>GSHMSEQFDFDLERILKTIKDKNCKKVGLQFPEGLKRQAINIAREIEEKTRANVIISGNPCFGACDIDTILAGSVDILFHF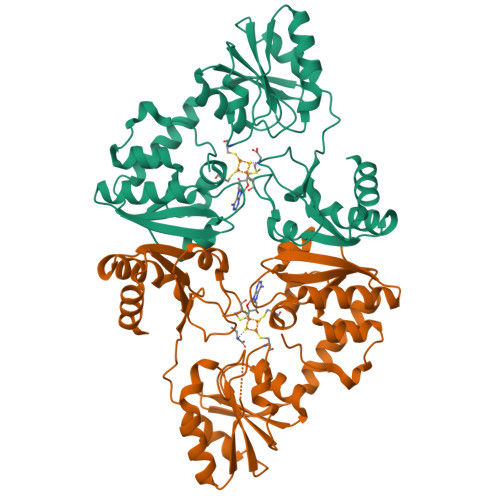GHAGMGEYENVVFIEARSNIDIIPAVKTALNLLKANRIGLITTVQHVHKLEEACKVIKEYGKECVIGKGDPRAIYPGQVLGCNFTAARVDCEEFIYIGSGIFHPLGVAIATKKRVIAADPFLNQAVEVSPERFLRKRGGYIAKATGAKIFGIIVSTKSGQYRMKLAQKLKEIADKHGKIGYIILMDLVTPEQLLAFKADAYVNTACPRITIDDAERFHAPVLTPQEFEIVLGERRWENMEMDEMIQ[2x]> MHHHHHHHHENLYFQGSRWKIIESYEGNSYTFIDPTQLPYNEKWEFPRNNLQFGKTLGAGAFGKVVEATAFGLGKEDAVLKVAVKMLKSTAHADEKEALMSELKIMSHLGQHENIVNLLGACTHGGPVLVITEYCCYGDLLNFLRRKRPPGLEYSYNPSHNPEEQLSSRDLLHFSSQVAQGMAFLASKNCIHRDVAARNVLLTNGHVAKIGDFGLARDIMNDSNYIVKGNARLPVKWMAPESIFDCVYTVQSDVWSYGILLWEIFSLGLN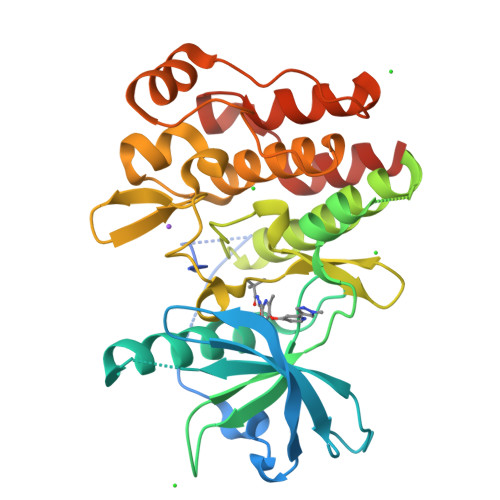PYPGILVNSKFYKLVKDGYQMAQPAFAPKNIYSIMQACWALEPTHRPTFQQICSFLQEQAQEDRRERD The capsaicin- and heat-activated receptor, TRPV1, has served as a model for deciphering lipid modulation, which is relevant to understanding how pro-algesic agents enhance channel activity in the setting of inflammatory pain. Identification of a pocket within the TRPV1 transmembrane core has provided initial clues as to how phosphoinositide lipids bind to and regulate the channel. Here we show that this regulatory pocket in rat TRPV1 can accommodate diverse lipid species, including the inflammatory lipid lysophosphatidic acid, whose actions are determined by their specific modes of binding. We captured several states of TRPV1 ranging from channels in which the VBP is empty to those bearing different bioactive lipids, including distinct phosphoinositide species, brominated phosphoinositide analogs and a pro-algesic lipid, lysophosphatidic acid (LPA). Together, our data show how the VBP accommodates a range of bioactive lipids and how occupancy of the site corresponds to the structural status of the pore.

To visualize the lipid–channel complex, we added LPA to nanodisc-reconstituted TRPV1 and determined a consensus cryo-EM map to a resolution of 3.0 Å. Through symmetry expansion and focused classification, we captured LPA bound within the vanilloid pocket in multiple stoichiometries, ranging from apo to all four subunits occupied. We thus refer to these structures as ‘empty’ to differentiate from the ‘apo’ structures, in which an endogenous lipid occupies the pocket. With resting and fully liganded structures representing closed and open configurations of the pore (S6) helices, respectively, we examined intermediate conformational states associated with substochiometric LPA binding (the four subunits are denoted as A through D in a counterclockwise orientation as viewed from the extracellular face).

>[4x]MEQRASLDSEESESPPQENSCLDPPDRDPNCKPPPVKPHIFTTRSRTRLFGKGDSEEASPLDCPYEEGGLASCPIITVSSVLTIQRPGDGPASVRPSSQDSVSAGEKPPRLYDRRSIFDAVAQSNCQELESLLPFLQRSKKRLTDSEFKDPETGKTCLLKAMLNLHNGQNDTIALLLDVARKTDSLKQFVNASYTDSYYKGQTALHIAIERRNMTLVTLLVENGADVQAAANGDFFKKTKGRPGFYFGELPLSLAACTNQLAIVKFLLQNSWQPADISARDSVGNTVLHALVEVADNTVDNTKFVTSMYNEILILGAKLHPTLKLEEITNRKGLTPLALAASSGKIGVLAYILQREIHEPECRHLSRKFTEWAYGPVHSSLYDLSCIDTCEKNSVLEVIAYSSSETPNRHDMLLVEPLNRLLQDKWDRFVKRIFYFNFFVYCLYMIIFTAAAYYRPVEGLPPYKLKNTVGDYFRVTGEILSVSGGVYFFFRGIQYFLQRRPSLKSLFVDSYSEILFFVQSLFMLVSVVLYFSQRKEYVASMVFSLAMGWTNMLYYTRGFQQMGIYAVMIEKMILRDLCRFMFVYLVFLFGFSTAVVTLIEDGKYNSLYSTCLELFKFTIGMGDLEFTENYDFKAVFIILLLAYVILTYILLLNMLIALMGETVNKIAQESKNIWKLQRAITILDTEKSFLKCMRKAFRSGKLLQVGFTPDGKDDYRWCFRVDEVNWTTWNTNVGIINEDPGNCEGVKRTLSFSLRSGRVSGRNWKNFALVPLLRDASTRDRHATQQEEVQLKHYTGSLKPEDAEVFKDSMVPGEK>MLILATLGSDKSVTTINAILTEIFTGLNPNKIIIFREDPQKKDIKGMEKALEYLGVNTLIEEKVIGEGIKLWREKIRNEEIDIFDITPGRKYMALSATYYSRAEEIRYVYLKDERE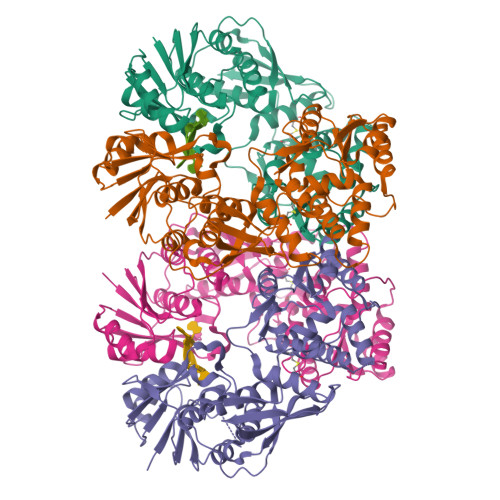GYNIFGYVPFEQLKVINVRIGDEIPYDPPLTQNVNEAESLLDVDSLRAFINILGLHGKVEINGIDLENPDQVEEICLFRSGKYKYEEEKDIIKEAERGSLFLADTNVYIRLGNRLRSLVYNRKYGFRLLSSKNTFNELYNHTAQDTQKIDENKVKFILGMLSYRSLHVPPITSQVRSSGDMGLINEALEIKKNVEDNVVLITADKALGLTAQSKGLRTIILSKVRKEIGEWDIGELLFCLSFYNDYRNGIRRMIEISLNGSKIAELHSYYHLQERRVKVRVVDKRYNYPKILEILSEILATADQAAAHHHHHH[4x]> TRDQNGTWEMESNENFEGYMKALDIDFATRKIAVRLTQTLVIDQDGDNFKFKTTSTFRNADVDFTVGVEFDEYTKSLDNRHVKALVTWEGDVLVCVQKGEKENRGWKKWIEGDKLYLELTCG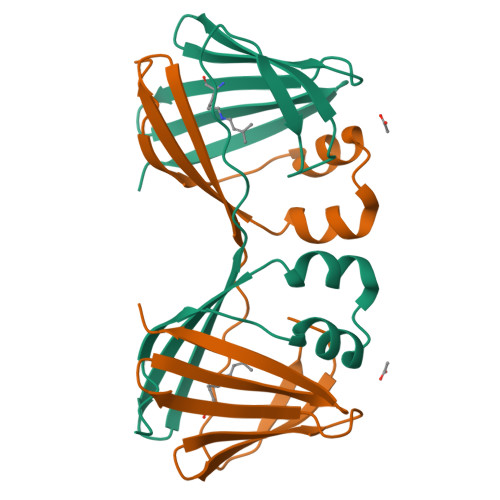DQVCRQVFKKK>[2x]SVSIGYLLVKHSQTDQEPMCPVGMNKLWSGYSLLYFEGQEK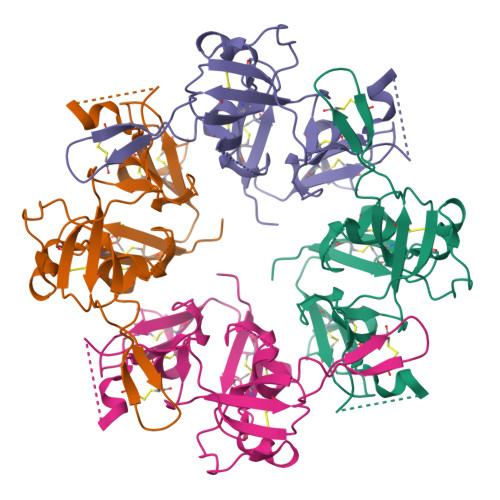AHNQDLGLAGSCLARFSTMPFLYCNPGDVCYYASRNDKSYWLSTTAPLPMMPVAEDEIKPYISRCSVCEAPAIAIAVHSQDVSIPHCPAGWRSLWIGYSFLMHTAAGDEGGGQSLVSPGSCLEDFRATPFIECNGGRGTCHYYANKYSFWLTTIPEQSFQGSPSADTLKAGLIRTHISRCQVCMKNL>MAHHHHHHAALRQPQVAELLAEARRAFREEFGAEPELAVSAPGRVNLIGEHTDYNQGLVLPMALELMTVLVGSPRKDGLVSLLTTSEGADEPQRLQFPLPTAQRSLEPGTPRWANYVKGVIQYYPAAPLPGFSAVVVSSVPLGGGLSSSASLEVATYTFLQQLCPDSGTIAARAQVCQQAEHSFAGMPCGIMDQFISLMGQKGHALLIDCRSLETSLVPLSDPKLAVLITNSNVRHSLASSEYPVRRRQCEEVARALGKESLREVQLEELEAARDLVSKEGFRRARHVVGEIRRTAQAAAALRRGDYRAFGRLMVESHRSLRDDYEVSCPELDQLVEAALAVPGVY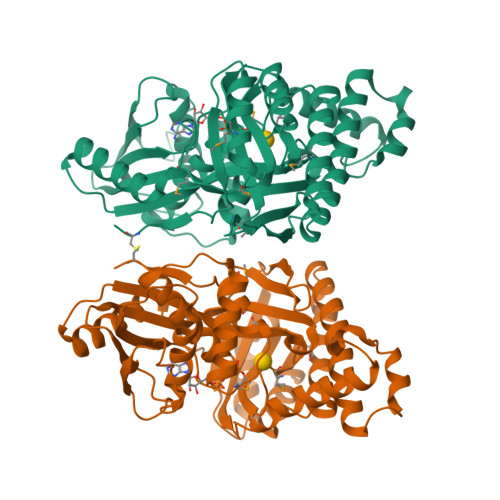GSRMTGGGFGGCTVTLLEASAAPHAMRHIQEHYGGTATFYLSQAADGAKVLCL[4x]>TGRPEWIWLALGTALMGLGALYFLVKGMGVSDPDAKKFYAITTLVPAIAFTMYLSMLLGYGLTMVPFGGEQNPIYWARYADWLFTTPLLLLDLALLVDADQGTILALVGADGIMIGTGLVGALTKVYSYRFVWWAISTAAMLYILYVLFFGFTSKAESMRPEVASTFKVLRNVTVVLWSAYPVVWLIGSEGAGIVPLNIETLLFMVLDVSAKVGFGLILLRSRAIFG[2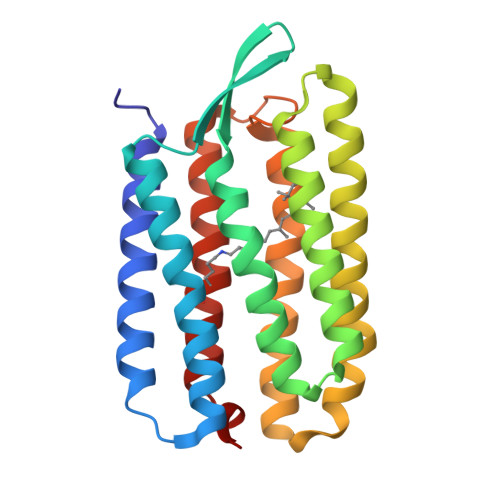x]> GPMFEARLVQGSILKKVLEALKDLINEACW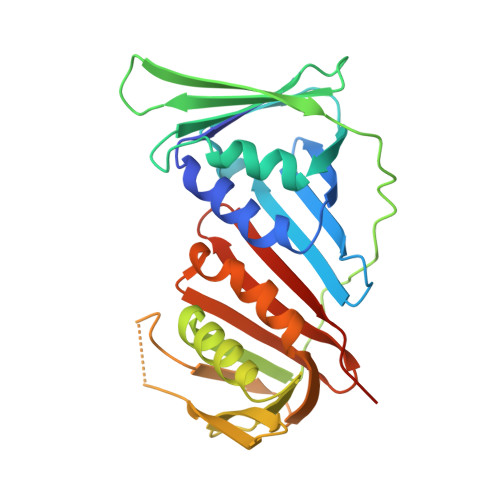DISSSGVNLQSMDSSHVSLVQLTLRSEGFDTYRCDRNLAMGVNLTSMSKILKCAGNEDIITLRAEDNADTLALVFEAPNQEKVSDYEMKLMDLDVEQLGIPEQEYSCVVKMPSGEFARICRDLSHIGDAVVISCAKDGVKFSASGELGNGNIKLSQTSNVDKEEEAVTIEMNEPVQLTFALRYLNFFTKATPLSSTVTLSMSADVPLVVEYKIADMGHLKYYLAPKIEDEEGS> CGSSTDPPVPNPYNTKEISLAAGLVQQTYCDSTEN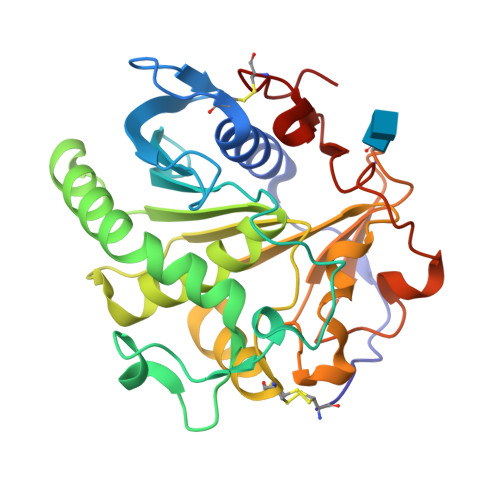GLKIGDSELLYTMGEGYARQRVNIYHSPSLGIAVAIEGTNLFSLNSDLHDAKFWQEDPNERYIQYYPKGTKLMHGFQQAYNDLMDDIFTAVKKYKKEKNEKRVTVIGHSLGAAVALLCAMDIELRMDGGLYKTYLFGLPRLGNCTFASFVDQKIGDKFHSIINGRDWVPTVPPRALGYQHPSDYVWIYPGNSTSAKLYPGQENVHGILTVAREFNNDDHQGIYFHTQIGAVRGECPAQVGAH The present study focuses on the PA14_16140 protein, i.e., the PA3732 (BacA) homolog in the PA14 strain. The role of BacA in rhamnolipid secretion, biofilm formation and virulence, was confirmed by phenotypic experiments with a bacA mutant. At a molecular level, quantitative proteomic studies revealed an accumulation of the BAC cognate partners by the bacA sessile mutant, suggesting a negative control of BacA toward the bac operon. Finally, a first crystallographic structure of BacA was obtained revealing a structure homologous to chaperones or/and regulatory proteins.

The domain search performed with Interpro database1 revealed that BacA is identified as a DUF 2170-containing domain protein (Pfam PF09938) belonging to the YjfI family. Nevertheless, the functional dimer conventionally described for the T3SS chaperone family does not correspond to this « asymmetric unit dimer » but is reconstituted by symmetry related molecules, issuing with two dimers each one being formed by crystallographic second order axis. The Tb-Xo4 molecule is localized at the interface of the two monomers present in the asymmetric unit, participating in the stabilization of the crystal packing, trapped by the N-terminus and Trp-39 of monomer A, by Glu-112 of monomer B interacting with the atom of terbium, and by Arg-136 of a symmetry-related monomer B. The 3D structures of the two monomers are very similar, with a two-layers alpha + beta mixed domain, and adopt the α-β-β-β-α-β-β-α topology characteristic of the T3SS chaperone family, with an average root-mean-square deviation (RMSD) of 0.6 Å on Cα for the 115 closest residues over the 139 amino-acids that have been crystallized. All the variability is localized at the N- and C-terminus and in the three loops linking the beta strands on the surface of the protein at the opposite side of the 3 alpha helices. Only 8 residues for each monomer, 3 at the N-terminus, 2 at the C-terminus and 3 in the loop 130–136 have not been constructed due to the absence of electron density (see dotted lines Figure 5B). Two residues present alternative positions, Glu-90 in monomer A (A-Glu-90) and His-155 in monomer B (B-His-155), these residues being localized at the biological dimer interface, in close proximity. One molecule of glycerol has been trapped in monomer A in the concave surface of the twisted six-stranded anti-parallel β-sheet in a pocket formed by the side chains of 4 residues (Tyr-72, Phe-84, Glu-95, Leu97). The location where is found this glycerol in molecule A corresponds to the region of interaction between the chaperone and the effector in the structure solved of the complex formed between the multi-cargo chaperone CesT and Tir from E. coli, Tir being the first translocated effector in the infected host cell via the T3SS.

>TEARVWNARSLAEALSGTELFSSGEAQIELIEGAEASLYVIMREYGDLPVFVAPQGEQIIVEALLWPESDVTDATAFNEEVLLSRQLFPLSSIGLLNLPGEERCYSMFGALSTTSSLASVLHEIETLAGNVIRATEVYAGYLKARA[2x]>[6x]MSLKITILAVGKLKEKY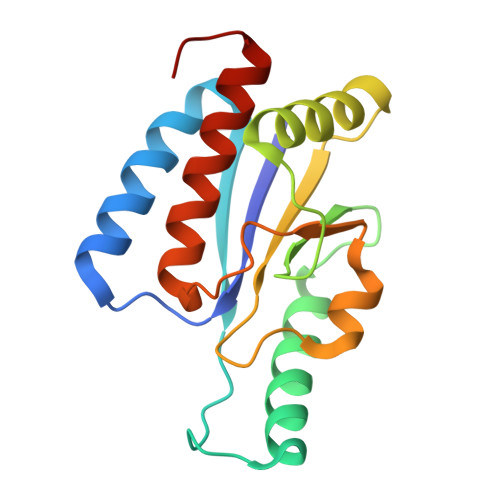WKQAIAEYEKRLGPYTKIDIIEVPDEKAPENMSDKEIEQVKEKEGQRILAKIKPQSTVITLEIQGKMLSSEGLAQELNQRMTQGQSDFVFVIGGSNGLHKDVLQRSNYALSFSKMTFPHQMMRVVLIEQVYRAFKIMRGEAYHK3-(2-aminoquinazolin-6-yl)-4-methyl-1-[3-(trifluoromethyl)phenyl]pyridin-2(1H)-one 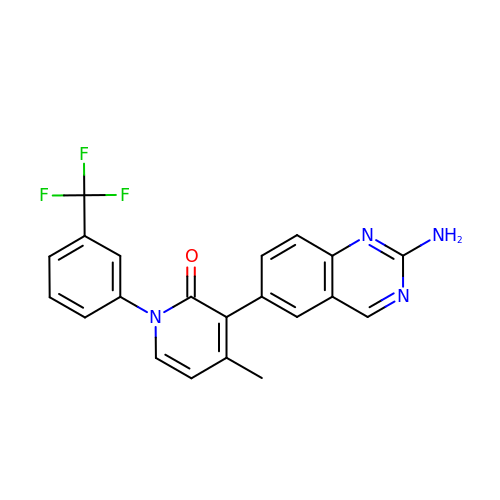| C21 H15 F3 N4 O | HXUZQEYFKAZBPX-UHFFFAOYSA-N> MNNQPQGTNSVPNSIGNIFSNIGTPSFNMAQIPQQLYQSLTPQQLQMIQQRHQQLLRSRLQQQQQQQQQTSPPPQTHQSPPPPPQQSQPIANQSATSTPPPPPAPHNLHPQIGQVPLAPAPINLPPQIAQLPLATQQQVLNKLRQQAIAKNNPQVVNAITVAQQQVQRQIEQQKGQQTAQTQLEQQRQLLVQQQQQQQLRNQIQRQQQQQFRHHVQIQQQQQKQQQQQQQHQQQQQQQQQQQQQQQQQQQQQQQQQQQQQQQQQQQQQGQIPQSQQVPQVRSMSGQPPTNVQPTIGQLPQLPKLNLPKYQTIQYDPPETKLPYPTYWSDKKADTDTLLYEQIIQRDKINKYSLIRETNGYDPFSIYGFSNKEYISRLWHTLKYYQDLKNTRMKSITSTSQKIPSASIWGNGYSGYGNGITNTTTRVIPQVEVGNRKHYLEDKLKVYKQAMNETSEQLVPIRLEFDQDRDRFFLRDTLLWNKNDKLIKIEDFVDDMLRDYRFEDATREQHIDTICQSIQEQIQEFQGNPYIELNQDRLGGDDLRIRIKLDIVVGQNQLIDQFEWDISNSDNCPEEFAESMCQELELPGEFVTAIAHSIREQ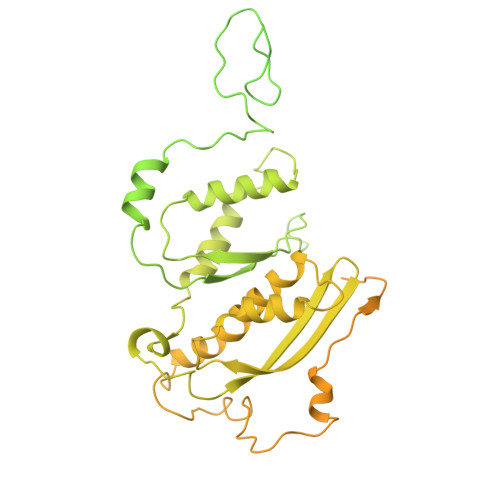VHMYHKSLALLGYNFDGSAIEDDDIRSRMLPTITLDDVYRPAAESKIFTPNLLQISAAELERLDKDKDRDTRRKRRQGRSNRRGMLALSGTSASNTSMNGVHNTVAAGNASSLPPGEILLPDIADIPRTFRTPVPSTLMPGGVDVGPSVESYELRNTTTYKSRPDRPKPVSPPCYIIDHIPGHSLLLSIKLPGKVNTKEEFAAAPNDTSSGTNAMLPSPESLKTKLNSNIRAGVTIPSIPNPIANHTVTNSPNPTLQPVIPGGAASKSVPTPSLPIAPPVAPHDSEATLLTNSNNGSSNNNTQNT> NDKLTLWTTPAPSPNCRLNAEKDAKLTLVLTKCGSQILATVSVL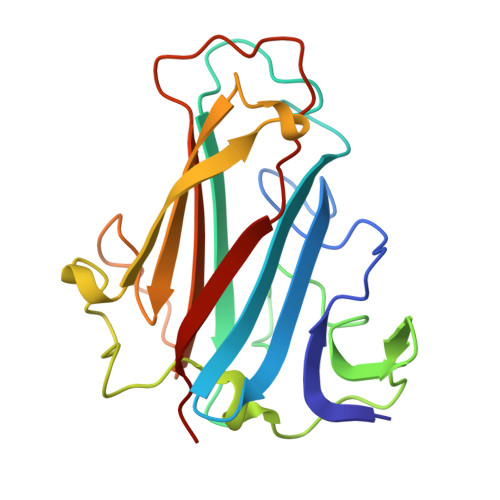AVKGSLAPISGTVQSAHLIIRFDENGVLLNNSFLDPEYWNFRNGDLTEGTAYTNAVGFMPNLSAYPKSHGKTAKSNIVSQVYLNGDKTKPVTLTITLNGTQETGDTTPSAYSMSFSWDWSGHNYINEIFATSSYTFSYIAQE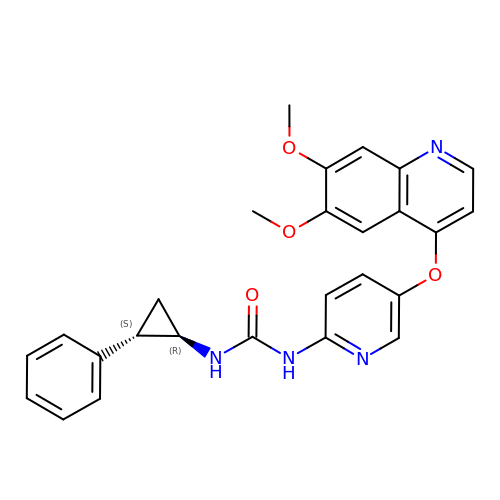1-{5-[(6,7-dimethoxyquinolin-4-yl)oxy]pyridin-2-yl}-3-[(1R,2S)-2-phenylcyclopropyl]urea | C26 H24 N4 O4 | MRWNNBQFJVSSHG-GHTZIAJQSA-N> MHHHHHHQIGWRREGIKYRRNELFLDVLESVNLLMSPQGQVLSAHVSGRVVMKSYLSG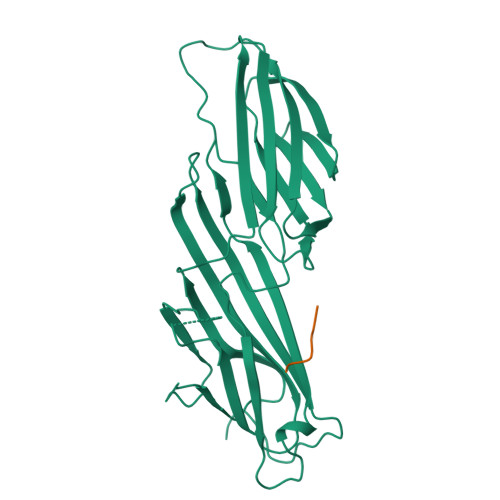MPECKFGMNDKIVIEKQGKGTADETSKSGKQSIAIDDCTFHQCVRLSKFDSERSISFIPPDGEFELMRYRTTKDIILPFRVIPLVREVGRTKLEVKVVIKSNFKPSLLAQKIEVRIPTPLNTSGVQVICMKGKAKYKASENAIVWKIKRMAGMKESQISAEIELLPTNDKKKWARPPISMNFEVPFAPSGLKVRYLKVFEPKLNYSDHDVIKWVRYIGRSGIYETRC;> DYQRLN>[24x]MSLGANIVSVEFIPVNVAATNWSENTVIVKVTDENGVYGLGEADGPPECMKAFSEIENEHKWLNNIKEAVIGRDPLEFRANYNR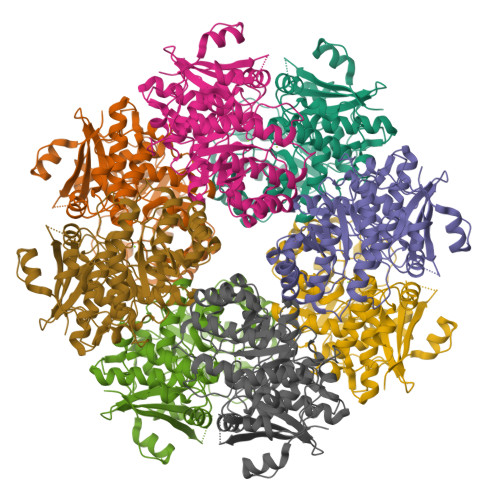MYDTTKWIGMRGLGLFAISGIDMALYDLAGKQLGVPAYKLMGGAQKAQLTPYFTLYPSVAADATLSEIVEAYKPLIAKAKERGAKAVKVCIIPNDKVSDKEIVAYLRELREVIGWDMDMMVDCLYRWTDWQKARWTFRQLEDIDLYFIEACLQHDDLIGHQKLAAAINTRLCGAEMSTTRFEAQEWLEKTGISVVQSDYNRCGGVTELLRIMDICEHHNAQLMPHNWKTGITAAAARHFGIVCHISEYVEYLHPDFWNGTLTQQLTLNEPKIIDGAIEVSDKPGLGIELNIEFVEQVTGHKFEGHHHHHH1-(4-chlorophenyl)-N-[2-(4-methoxyphenyl)-5,5-bis(oxidanylidene)-4,6-dihydrothieno[3,4-c]pyrazol-3-yl]cyclopentane-1-carboxamide | C24 H24 Cl N3 O4 S | 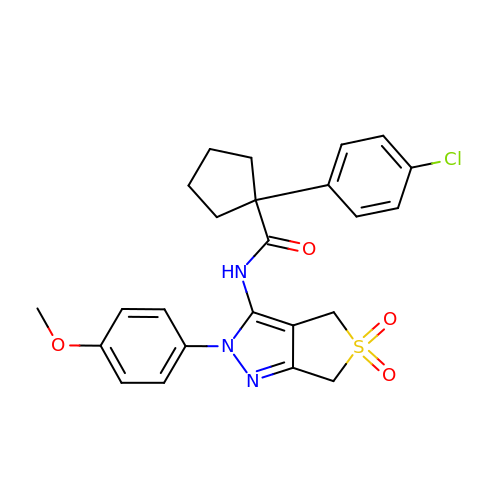DDCUCVXSGYHWRJ-UHFFFAOYSA-N>[4x]MRGSHHHHHHGSKFCRFGQRGQEKPGIIDADGNIRDLSGVVPELTIDALAAAKGADIALLPLVEGE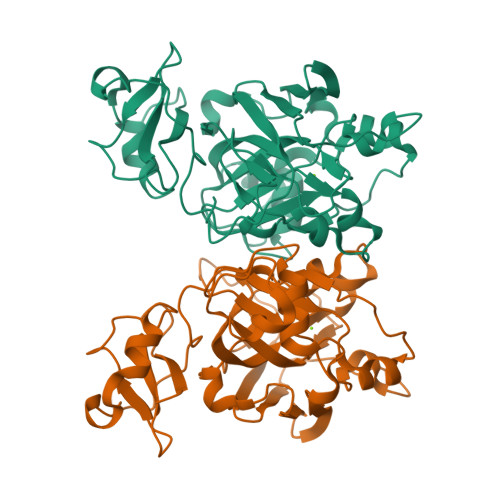PRYGVPVKGIGKIVAIGLNYEDHAIESNLPIPTEPMMFMKALSSLNGPNDEVVLPKNSTHGDWEVELGVVIGETCRFVSEDEALSKVAGYVLVNDVSERFNQKQRGTQWSKGKGHDTFCPVGPWLVTPDEVGDPQDLDVHLDVNGERMQTGNTKTMIFNVAQLISYVSEYITLYPGDLMITGTPPGVGEGKKPQAIYLKAGDVMELGIEKLGTQRQQVSEWRHLGDEVFG>METDNVELAQSKRKVVLAEQGSFYIGGRTVTGPGKFDPSKPVIPYSNEGATFYINQMYVNFQAPVRPRGLPLVFWHGGGLTGHIWESTPDGRPGFQTLFVQDRHTVYTIDQPGRGRGNIPTFNGPFGQLEEESIVNTVTGNSSKEGAWVRDRLGPAPGQFFENSQFPRGYEDNYFKEMGFSPSISSDEIVDAVVKLVTHIGPCVLVTHAASGVLGMRVATHAKNVRGIVAYEPATSIFPKGKVPEIPPLADKKSQIFPPFEIQESYFKKLAKIPIQFVFGDNIPKNPKSAYWFLDWWRVTRYAHSLSLEAINKLGGQASLLDLPTAGLRGNTAFPFTDRNNVQVASLLSDFLGKHGLDQNESLEHHHHHH[2x]

SulE, an esterase, which detoxifies a variety of sulfonylurea herbicides through de-esterification, provides an attractive approach to remove environmental sulfonylurea herbicides and develop herbicide-tolerant crops. SulE catalyzes the de-esterification of a variety of sulfonylurea herbicides, such as MM, BM, SM, TM, TrM, EM, and CE, to the corresponding herbicidal-inactive parent acid. The structures show that SulE is a dimer with a lid loop in a domain-swapped β-hairpin covering the active site from the opposing monomer. SulE shows a similar catalytic triad consisting of Ser209, His333, and Glu232 at its active site.

To elucidate the catalytic mechanism of SulE, we solved the crystal structures of wild-type SulE in complex with CA, mutant S209A in complex with MM, and mutant S209A/H333A in complex with MM, SM, TM, TrM, EM, BM, and CE in the range of 1.29–1.63 Å. Seven sulfonylureas bind in a similar manner in the spacious active pocket of SulE. In the other six substrate-bound complex structures of S209A/H333A, clear electron density also could be observed for SM, AM, CE, and TrM, but the density for BM and TM were relatively poor. Upon binding to SulE, the seven substrates adopted a similar conformation with a bend at the sulfonyl group, making the aromatic ring and heterocycle nearly perpendicular to each other. In the six structures of S209A/H333A bound to MM, EM, TrM, CE, SM, and BM, the ester O atom is hydrogen-bonded with the main chain nitrogen atoms of Gly78 and Ala210, forming an oxyanion hole. Superimposing the seven sulfonylurea complex structures showed that residues involved in the formation of the active pocket are almost completely superimposed, indicating that these residues do not undergo conformational changes when binding to different ligands. Furthermore, the aromatic ring of these seven sulfonylureas is also well-superposed, indicating that this moiety strongly interacted with SulE. However, their sulfonylurea bridge and heterocyclic moiety are not well superimposed except for MM and CE, implying that this moiety is not tightly anchored on SulE.> DSLDEQRSRYAQIKQAWDNRQMDVVEQMMPGLKDYPLYPYLEYRQITDDLMNQPAVTVTNFVRANPTLPPARTLQSRFVNELARREDWRGLLAFSPEKPGTTEAQCNYYYAKWNTGQSEEAWQGAKELWLTGKSQPNACDKLFSVWRASGKQDPLAYLERIRLAMKAGNTGLVTVLAGQMPADYQTIASAIISLANNPNTVLTFARTTGATDFTRQMAAVAFASVARQDAENARLMIPSLAQAQQLNEDQIQELRDIVAWRLMGNDVTDEQAKWRDDAIMRSQSTSLIERRVRMALGTGDRRGLNTWLARLPMEAKEKDEWRYWQADLLLERGREAEAKEILHQLMQQRGFYPMVAAQRIG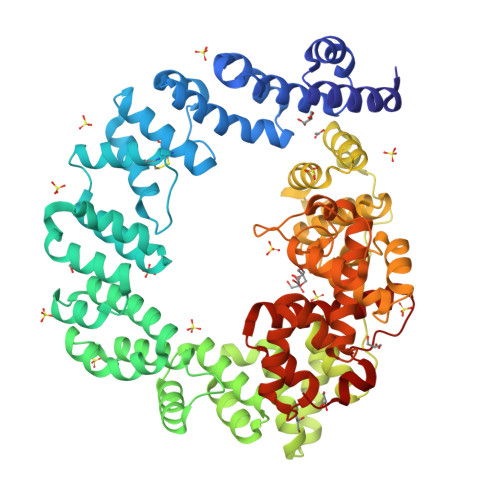EEYELKIDKAPQNVDSALTQGPEMARVRELMYWNLDNTARSEWANLVKSKSKTEQAQLARYAFNNQWWDLSVQATIAGKLWDHLEERFPLAYNDLFKRYTSGKEIPQSYAMAIARQESAWNPKVKSPVGASGLMQIMPGTATHTVKMFSIPGYSSPGQLLDPETNINIGTSYLQYVYQQFGNNRIFSSAAYNAGPGRVRTWLGNSAGRIDAVAFVESIPFSETRGYVKNVLAYDAYYRYFMGDKPTLMSATEWGRRY>GHMGKPDISAKDLRNIMYDHLPGFGTAFHQLVQVICKLGKDSNSLDIIHAEFQASLAEGDSPQCALIQITKRVPIFQDAAP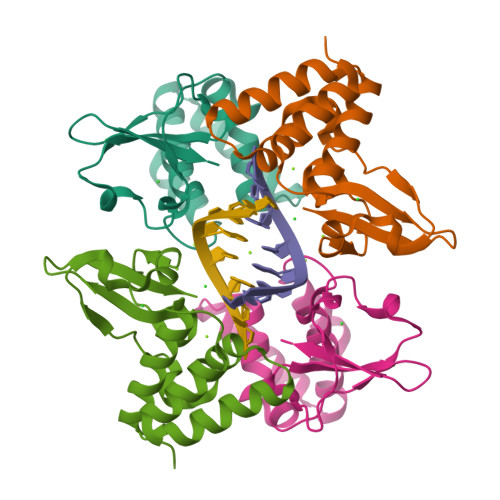PVIHIRSRGDIPRACQKSLRPVPPSPKIDRGWVCVFQLQDGKTLGLKI[2x]> MHFSIPETESRSGDSGGSAYVAYNIHVNGVLHCRVRYSQLLGLHEQLRKEYG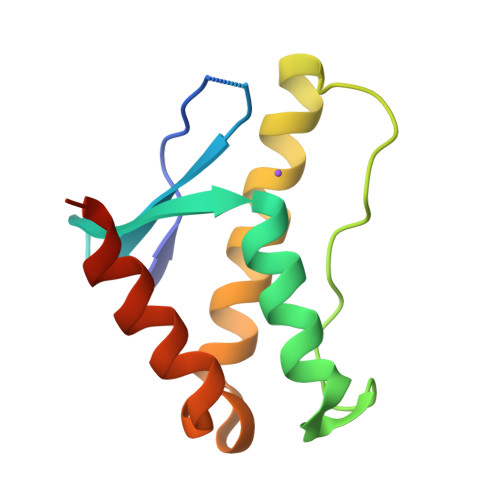ANVLPAFPPKKLFSLTPAEVEQRREQLEKYMQAVRQDPLLGSSETFNSFLRRAQQEAHHHHHH> YDSRSSGVHDVAPRDGVDFMYEGPQQVLPGAHPLPLFHPDNSVTRPPVSPYLPSPQRPHPYFTTELPELPHFQTTRPIVYTVGTMKQRIVAPVFDLANNVTHTRELDPFIFGFYPETEEMAKNLSYWLVRCQNFSSKWDYENREIWRKAKKNWPNTGMGMARVGDRKNHAHPWGAHSKPVKPWNLLMPTMDVKTWSKSNRMLVTLKMLQGKLQIVERLTLPEPTQEAYLQLCRTMGWDVRHKGGGALFMDGGSRLTPSSEYDRAFFFGSFFNGRNKLVRPTLLCDEPYDYNRTSSKARTKGPKGQKNPIPINRFNAYDALTHDTLIITEGALLQLEDEMYTHKLAMLPPHIRAQLPERGFLDSEVLGDVPPALQTVQMEAAARTEEAEQA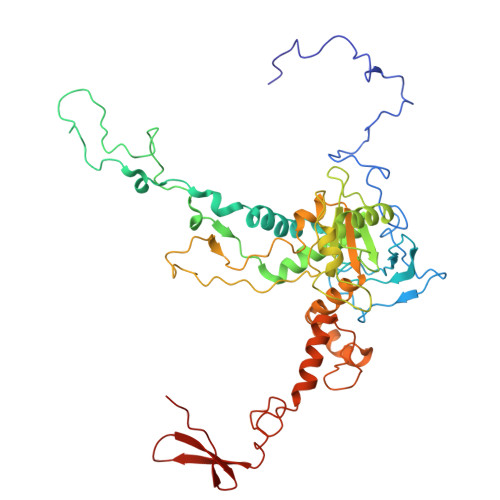MYAPYYDNPYHPWQDEGEASYAVDAVEGTVQRYIKSRKTSWAMLS>MKRIKCNKVRTVTEIVNSDEKIQKTYELAEFDLKNLSSLESYETLKIKLALSKYMAMLSTLEMTQPLLEIFRNKADTRQIAAVVFSTLAFIHNRFHPLVTNFTNKMEFVVTETNDTSIPGEPILFTENEGVLLCSVDRPSIVKMLSREFDTEALVNFENDNCNVRIAKTFGASKRKNTTRSDDYESNKQPNYDMDLSDFSITEVEATQYLTLLLTVEHAYLHYYIFKNYGVFEYCKSLTDHSLFTNKLRSTMSTKTSNLLLSKFKFTIEDFDKINSNSVTSGFNIYNFNK[6x];>MSAIALYLEINKLRLKIDEPMQLAIWPQLFPLLCDEHQSVQLNTDVLINFMMHVARKSQNTILNNNAAIASQYAAGNADVVAAPASAQPTPRPVINLFARANAAAPAQPSEELINMRRYRNAARKLIHHYSLNSTSSTEYKISDVVMTMIFLLRSEKYHSLFKLLETTFDDYTCRPQMTQVQTDTLLDAVRSLLEMPSTTIDLTTVDIMRSSFARCFNSPIMRYAKIVLLQNVALQRDKRTTLEELLIERGEKIQMLQPQQYINSGTEIPFCDDAEFLNRLLKHIDPYPLSRMYYNAANTMFYTTMENYAVSNCKFNIEDYNNIFKVMENIRKHSNKNSNDQDELNIYLGVQSSNAKRKKY[6x];>[2x]MASSLQSKWICLRLNDAIIKRHVLVLSEYADLKYLGFEKYKFFEYVIFQFCNDPQLCKIIENNYNYCMQIFKAPADDMRDIRHNIKRAFKTPVLGHMCVLSNKPPMYSFLKEWFLLPHYKVVSLKSESLTWGFPHVVVFDLDSTLITEEEQVEIRDPFVYDSLQELHEMGCVLVLWSYGSRDHVAHSMRDVDLEGYFDIIISEGSTVQEERSDLVQNSHNAIVDYNLKKRFIENKFVFDIHNHRSDNNIPKSPKIVIKYLSDKNVNFFKSITLVDDLPTNNYAYDFYVKVKRCPTPVQDWEHYHNEIIQNIMDYEQYFIK;>MSGGGNLLTLERDHFKYLFLTSYFDLKDNEHVPSEPMAFIRNYLNCTFDLLDDAVLMNYFNYLQSMQLKHLVGSTSTNIFKFVKPQFRFVCDRTTVDILEFDTRMYIKPGTPVYATNLFTSNPRKMMAFLYAEFGKVFKNKIFVNINNYGCVLAGSAGFLFDDAYVDWNGVRMCAAPRLDNNMHPFRLYLLGEDMAKHFVDNNILPPHPSNAKTRKINNSMFMLKNFYKGLPLFKSKYTVVNSTKIVTRKPNDIFNEIDKELNGNCPFIKFIQRDYIFDAQFPPDLLDLLNEYMTKSSIMKIITKFVIEENPAMSGEMSREIILDRYSVDNYRKLYIKMEITNQFPVMYDHESSYIFVSKDFLQLKGTMNAFYAPKQRILSILAVNRLFGATETIDFHPNLLVYRQSSPPVRLTGDVYVVDKNEKVFLVKHVFSNTVPAYLLIRGDYESSSDLKSLRDLNPWVQNTLLKLLIPDSVQ[2x];>MALVPVGMAPRQMRVNRCIFASIVSFDACITYKSPCSPDAYHDDGWFICNNHLIKRFKMSKMVLPIFDEDDNQFKMTIARHLVGNKERGIKRILIPSATNYQDVFNLNSMMQAEQLIFHLIYNNENAVNTICDNLKYTEGFTSNTQRVIHSVYATTKSILDTTNPNTFCSRVSRDELRFFDVTNARALRGGAGDQLFNNYSGFLQNLIRRAVAPEYLQIDTEELRFRNCATCIIDETGLVASVPDGPELYNPIRSSDIMRSQPNRLQIRNVLKFEGDTRELDRTLSGYEEYPTYVPLFLGYQIINSENNFLRNDFIPRANPNATLGGGAVAGPAPGVAGEAGGGIAV[8x];>[6x]MNDSNSLLITRLAAQILSRNMQTVDVIVDDKTLSLEEKIDTLTSMVLAVNSPPQSPPRVTSSDLAASIIKNNSKMVGNDFEMRYNVLRMAVVFVKHYPKYYNETTAGLVAEIESNLLQYQNYVNQGNYQNIEGYDSLLNKAEECYVKIDRLFKESIKKIMDDTEAFEREQEAERLRAEQTAANALLERRAQTSADDVVNRADANIPTAFSDPLPGPSAPRYMYESSESDTYMETARRTAEHYTDQDKDYNAAYTADEYNSLVKTVLLRLIEKALATLKNRLHITTIDQLKKFRDYLNSDADAGEFQIFLNQEDCVILKNLSNLASKFFNVRCVADTLEVMLEALRNNIELVQPESDAVRRIVIKMTQEIKDSSTPLYNIAMYKSDYDAIKNKNIKTLFDLYNDRLPINFLDTSATSPVRKTSGKRSAEDDLLPTRSSKRANRPEINVISSEDEQEDDDVEDVDYEKESKRRKLEDEDFLKLKALEFSKDIVNEKLQKIIVVTDGMKRLYEYCNCKNSLETLPSAANYGSLLKRLNLYNLDHIEMNVNFYELLFPLTLYNDNDNSDKTLSHQLVNYIFLASNYFQNCAKNFNYMRETFNVFGPFKQIDFMVMFVIKFNFLCDMRNFAKLIDELVPNKQPNMRIHSVLVMRDKIVKLAFSNLQFQTFSKKDKSRNTKHLQRLIMLMNANYNVI;>[2x]MECPFQIQVCISDRFFAFPHNLVEPQSDVGNKLIENLIVYVPTDDDRLYIDKKQFPKFNSVLVYRHEHDVNIDSRSPKKTASATIVYWNPLVPITEIGAGETRVFSVLLTNNLFYCNTMIVHHENPKCPIEFTYPETDMQSACSALLKNRNGQSVPPPIKSNLRPIACEIPLSHFKELVESNDFLLCFNLETSTMVKILSLKRIFCIFQYRKQPARYVINLPHEEIDNLYNKLNWERTRRLMKGDVPSNCATVNRSSLKYIKQAQSLLGIPDYSQTVVDFVKMFQKIIFPYQLVPNVIIKLNNFDQMVSSAPNKAEPYKKIRLFCKNDSIAISSSGIVPINMPDFSPPNTFDYSDYANRTNINFVTQRVLTDGGFSSGITVTPVKYNYYL

The most well-studied baculovirus is Autographa californica multiple nucleopolyhedrovirus (AcMNPV). Baculoviruses have their large circular dsDNA genome packaged into an enveloped rod-shaped nucleocapsid. The BV nucleocapsid structure consists of three parts, a central helical sheath containing the viral genome, an apical cap and a basal structure attached to both extremities of the helical sheath. Herein, we report high-resolution cryo-electron microscopy (cryo-EM) structures of the BV nucleocapsid combined with de novo modeling and Alphafold predictions.

The entire basal structure was determined to 5.2 Å resolution (applying a C7 symmetry), delineating two different symmetrical rings: an outer one with C14 symmetry surrounding an inner one with C7 symmetry. 3D refinements focused on these individual rings with their respective symmetries applied, resulted in higher resolution structures, 4.1 Å for C14 and 3.4 Å for C7 rings. The baffling distinction between the two cap complexes is that the anchor-2 rings, which are very similar to each other, interact with innermost components displaying different cyclic symmetries. In the apical cap, anchor-2 connects to the C2 symmetric part of the portal leading to a C14 to C2 mismatch while in the basal structure, it connects to the C7 plug producing a C14 to C7 symmetry mismatch. A major difference between the anchor-2 complexes in the apical and basal structures is the presence of Ac98 in the basal anchor-2, which interacts exclusively with Ac144 from the lowermost Ac101/Ac144 module. The inner part of the basal structure has a C7 symmetry and functions as a plug closing the void created by the peripheric C14 anchor complex.>DENSKKTQELVEKLPHEVLELYKNVGGEIYITDKRLTQHEELSDSSHKDMFIVSSEGKSFPLREHFVFAKGGKEPSLIIHAEDYASHLSSVEVYYELGKAIIRDTFPLNQKELGNPKFINAINEVNQQKEGKGVNAKADEDGRDLLFGKELKKNLEHGQLVDLDLISGNLSEFQHVFAKSFALYYEPHYKEALKSYAPALFNYMLELDQMRFKEISDDVKEKNKNVLDFKWYTRKAESWGVQTFKNWKENLTISEKDIITGYTGSKYDPINEYLRKYDGEIIPNIGGDLDKKSKKALEKIENQIKNLDAALQKS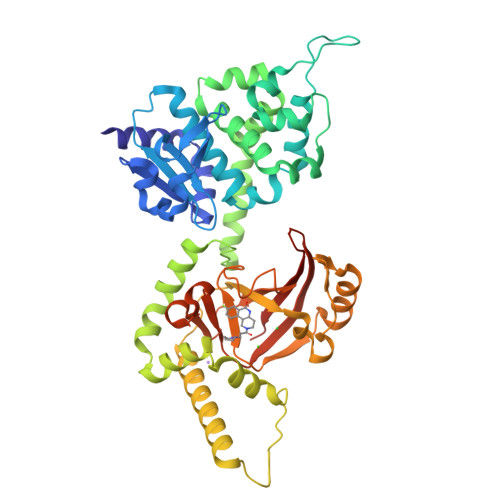KITENLIVYRRVSELQFGKKYEDYNLRQNGIINEEKVMELESNFKGQTFIQHNYMSTSLVQDPHQSYSNDRYPILLEITIPEGVHGAYIADMSEYPGQYEMLINRGYTFKYDKFSIVKPTREEDKGKEYLKVNLSIYLGNHHHHHH[2x]>[3x]MKQCAHTKVWQTIVAEAREQAEQEPMLASFYHATIIKHDSLKAALSYILANRLNTASMPAMAVREVIEEAFAADPSISEAAACDICATVNRDPAVSMYSMPLLYLKGYHAL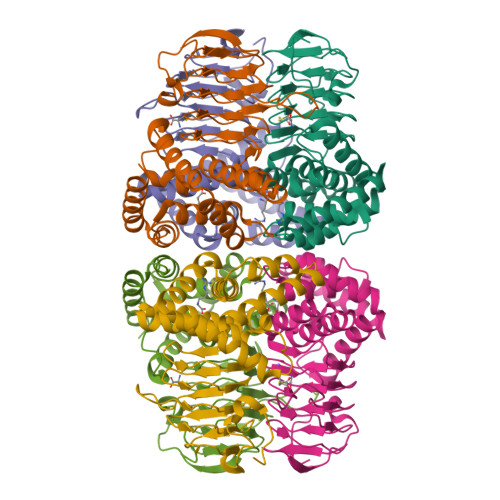QGYRVANWLWRQGRKALATYFQNQISVACQVDIHPAARIGRGIMLDHATGIVIGETAVVEDDVSILQDVTLGGTGKECGDRHPKIREGVMIGAGAKILGNIEVGEGAKIGSGSVVLQAVPPHTTVAGVPARIVGRPQSDKPSLDMDQQFNGRSQTFIGGDGILEHHHHHH> AMAMSSLPVAAVLPELLTALDCAPQVLLSAPTGAGKSTWLPLQLLAHPGINGKIILLEPRRLAARNVAQRLAELLNEKPGDTVGYRMRAQNCVGPNTRLEVVTEGVLTRMIQRDPELSGVGLVILDEFHERSLQADLALALLLDVQQGLRDDLKLLIMSATLDNDRLQQMLPEAPVVISEGRSFPVERRYLPLPAHQRFDDAVAVATAEMLRQESGSLLLFLPGVGEIQRVQEQLASRIGSDVLLCPLYGALSLNDQRKAILPAPQGMRKVVLATNIAETSLTIEGIRLVVDCAQERVARFDPRTGLTRLITQRVSQASMTQRAGRAGRLEPGISLHLIAKEQAERAAAQSEPEILQSDLSGLLMELLQWGCSDPAQMSWLDQPPVVNLLAAKRLLQMLGALEGERLSAQGQKMAALGNDPRLAAMLVSAKNDDEAATAAKIAAILEEPPRMGNSDLGVAFSRNQPAWQQRSQQLLKRLNVRGGEADSSLIAPLLAGAFADRIARRRGQDGRYQLANGMGAMLDANDALSRHEWLIAPLLLQGSASPDARILLALLVDIDELVQRCPQLVQQSDTVEWDDAQGTLKAWRRLQIGQLTVKVQPLAKPSEDELHQAMLNGIRDKGLSVLNWTAEAEQLRLRLLCAAKWLPEYDWPAVDDESLLAALETWLLPHMTGVHSLRGLKSLDIYQALRGLLDWGMQQRLDSELPAHYTVPTGSRIAIRYHEDNPPALAVRMQEMFGEATNPT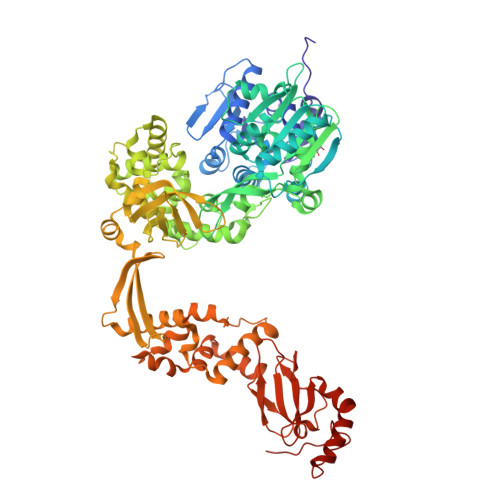IAQGRVPLVLELLSPAQRPLQITRDLSDFWKGAYREVQKEMKGRYPKHVWPDDPANTAPTRRTKKYS> SNAMLFDEKEILAITRWAKLYANQSPDRILLGSNDIPPEYRAAVATQIELWPRLRNKLPQWAGISSLYIPSRLSLEQSSGAVTSSYKSRFIREGTKVVDLTGGLGIDFIALMSKASQGIYIERNDETAVAARHNIPLLLNEGKDVNILTGDFKEYLPLIKTFHPDYIYVDPARRSGADKRVYAIADCEPDLIPLATELLPFCSSILAKLSPMIDLWDTLQSLLHVQELHVVAAHGEVKELLVRMSLNEATIPPEKVPIHAINLLLEDTVIPFIFTMEEERSISIPYTDSIDKYVYEPHTALLKAGAFKTVAYRLGLRKLHPNSHLYTSEAYESAFPGRTFVLEEIIPFSTSVLKQLRKVVPQASISCRNFPLSPIELRQRSKM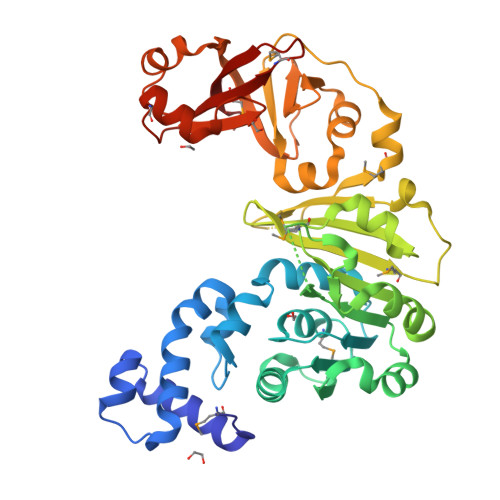ADGGEKTLMGTTMADGKKVLLLLRKAE> GIGKFLHSAKKFGKAFVGEIMNS

Magainin-2 (Mag-2) is a well-studied AMP, originally isolated from frog skin, consisting of 23 residues and carrying a net positive charge of + 3 (sequence: GIGKFLHSAKKFGKAFVGEIMNS). It has been shown to effectively kill MDR strains of Escherichia coli, Klebsiella pneumoniae, Pseudomonas aeruginosa or Staphylococcus aureus. Like other AMPs, Mag-2 interacts with negatively charged components such as LPS, LTA, and bacterial cytoplasmic membranes, leading to membrane destabilization. In this paper, we focus on Mag-2 which had previously also been shown to exhibit discrete conductivity steps when embedded in planar lipid membranes.

While we failed to obtain crystals of Mag-2 in the presence of DDM, we successfully achieved crystallisation in the presence of a Mag-2:DPC ratio of 1:3.5 (4 mM Mag-2 and 0.5% DPC = (14 mM)). These crystals diffracted to atomic resolution, revealing a α-helical three-dimensional structure in which two antiparallel monomers associate to form a dimer via a prominent hydrophobic interface. One monomer was observed in the asymmetric unit. The structure of the monomer displayed a single α-helix comprising all residues (Gly1-Asn22) except Ser23, which was not ordered. Notably, the aromatic side chains formed a long-range connected network of five aromatic interactions arranged in a phenylalanine zipper (Phe5/Phe16’, Phe5/Phe12’, Phe12/Phe12’, Phe12/Phe5´, Phe16/Phe5’). The opposite side of the dimer was dominated by hydrophilic residues, including eight lysines (Lys4/Lys4’, Lys10/Lys10’, Lys11/Lys11’ and Lys14/Lys14’), two histidines (His7/His7’) and two glutamates (Glu19/Glu19’) at the C-terminal end of the peptide contributing to an overall charge of + 6. Upon further examination of the crystallographic environment of the dimer, we noticed that a hexameric channel-like structure based on three peptide dimers and threefold symmetry with reasonable peptide-peptide interfaces could be constructed (PISA´s resulting interface of 4596 Å2). The outer overall dimensions of this hexameric channel were 3.5 nm in height and 4.5 nm in width, and a very narrow central pore of approximately 0.35 nm. Within the pore, two layers of adjacent positive charges, mainly Lys10 and His7, were located, while residues 10–22 did not significantly contribute to the inner pore architecture. Specifically, we demonstrated the ability of the Mag-2 channel to allow the pass of chloride anions, being non-permeable to potassium cations.> PKLLNKFDKTIKAELDAAEKLRKRGKIEEAVNAFKELVRKYPQSPRARYGKAQCEDDLAEKRRSNEVLRGAIETYQEVASLPDVPADLLKLSLKRRSDRQQFLGHMRGSLLTLQRLVQLFPNDTSLKNDLGVGYLLIGDNDNAKKVYEEVLSVTPNDGFAKVHYGFILKAQNKIAESIPYLKEGIESGDPGTDDGRFY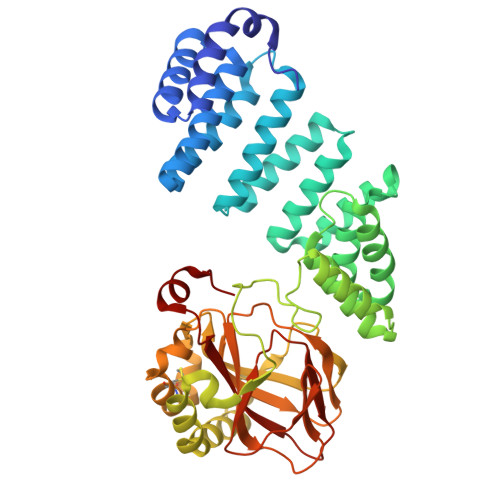FHLGDAMQRVGNKEAYKWYELGHKRGHFASVWQRSLYNVNGLKAQPWWTPKETGYTELVKSLERNWKLIRDEGLAVMDKAKGLFLPEDENLREKGDWSQFTLWQQGRRNENACKGAPKTCTLLEKFPETTGCRRGQIKYSIMHPGTHVWPHTGPTNCRLRMHLGLVIPKEGCKIRCANETKTWEEGKVLIFDDSFEHEVWQDASSFRLIFIVDVWHPELTPQQRRSLPAI> SPFKPRNYQLELALPAMKGKNTIICAPTGCGKTFVSLLICEHHLKKFPQGQKGKVVFFANQIPVYEQNKSVFSKYFERHGYRVTGISGATAENVPVEQIVENNDIIILTPQILVNNLKKGTIPSLSIFTLMIFDECHNTSKQHPYNMIMFNYLDQKLGGSSGPLPQVIGLTASVGV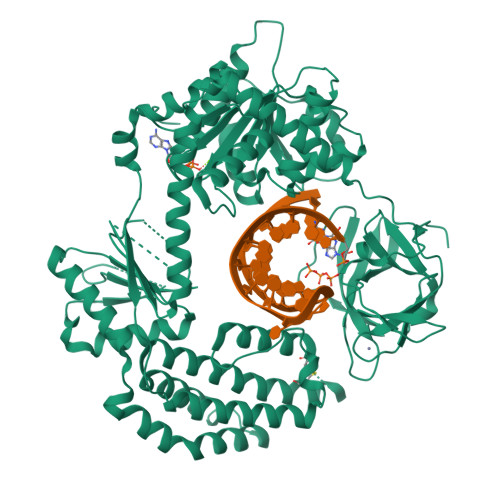GDAKNTDEALDYICKLCASLDASVIATVKHNLEELEQVVYKPQKFFRKVESRISDKFKYIIAQLMRDTESLAKRICKDLENLSQIQNREFGTQKYEQWIVTVQKACMVFQMPDKDEESRICKALFLYTSHLRKYNDALIISEHARMKDALDYLKDFFSNVRAAGFDEIEQDLTQRFEEKLQELESVSRDPSNENPKLEDLCFILQEEYHLNPETITILFVKTRALVDALKNWIEGNPKLSFLKPGILTGRGKTNQNTGMTLPAQKCILDAFKASGDHNILIATSVADEGIDIAQCNLVILYEYVGNVIKMIQTRGRGRARGSKCFLLTSNAGVIEKEQINMYKEKMMNDSILRLQTWDEAVFREKILHIQTHEKFIRDSQEKPKPVPDKENKKLLCRKCKALACYTADVRVIEDCHYTVLGDAFKECFVSRPHPKPKQFSSFEKRAKIFCARQNCSHDWGIHVKYKTFEIPVIKIESFVVEDIATGVQTLYSKWKDFHFEKIPFDPAEMSK>MKEKVVSLAQDLIRRPSISPNDEGCQQIIAERLEKLGFQIEWMPFNDTLNLWAKHGTSEPVIAFAGHTDVVPTGDENQWSSPPFSAEIIDGMLYGRGAADMKGSLAAMIVAAEEYVKANPNHKGTIALLITSDEEAT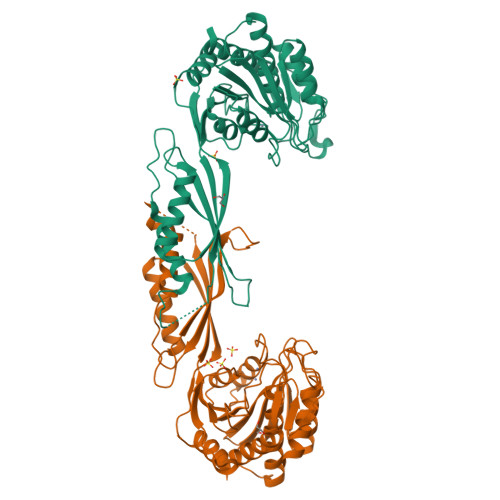AKDGTIHVVETLMARDEKITYCMVGEPSSAKNLGDVVKNGRRGSITGNLYIQGIQGHVAYPHLAENPIHKAALFLQELTTYQWDKGNEFFPPTSLQIANIHAGTGSNNVIPAELYIQFNLRYCTEVTDEIIKQKVAEMLEKHNLKYRIEWNLSGKPFLTKPGKLLDSITSAIEETIGITPKAETGGGTSDGRFIALMGAEVVEFGPLNSTIHKVNECVSVEDLGKCGEIYHKMLVNLLDS[2x]> MHHHHHHITSLYKKAGSEFALDSSKLEAIYATSEADRDYKENAVDGDENTIWHSAYQAADKLPVSITIKLDKA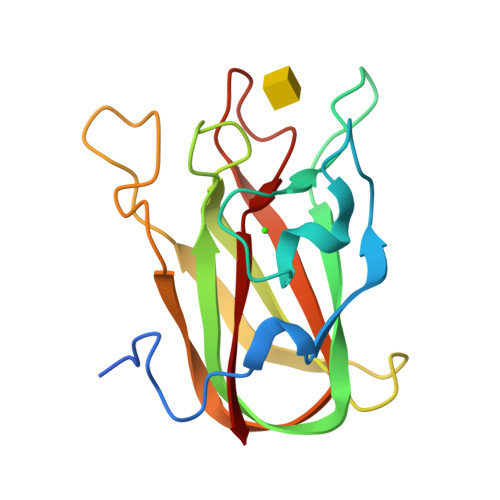YDLNQIDYLPRQNSRNGHVTEYKIETSLDNENWTEVRTGNLEVNEAGNALANRGYNPIRFNTINAQYLRFTALKTLGDTNNKYASAAELVFYGK>MGSSHHHHHH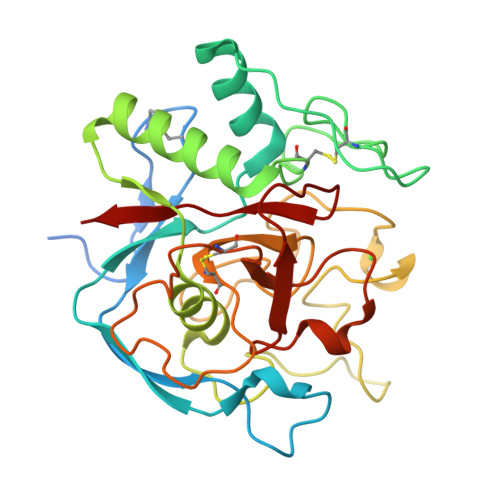SQDLEVLFQGPGSDEAKKPGTVFKDCKDCPEMVVLPAGSFTMGTPDDEVGRQPDEGPLHDVTFAKPFAISRYQVTAGELDAYLKATGVKLADGDTRPGRECIAGKPRYQQGPRQPAVCVDYNDVKNYAAWLSKKTGKRYRMLSEAEREYGARAGSAGPFPFPFDEGKEYSIAKHANTYGASDGYNFTSPVGSFPPNAFGVYDMHGNVYEWVADCWHDHYNGAPSDGSAWMEEKCELVQIRGNDWGEPPIFSRSGNRNNAAPSDRGDWIGFRVAREL[2x]> MSDILQELLRVSEKAANIARACRQQETLFQLLIEEKKEGEKNKKFAV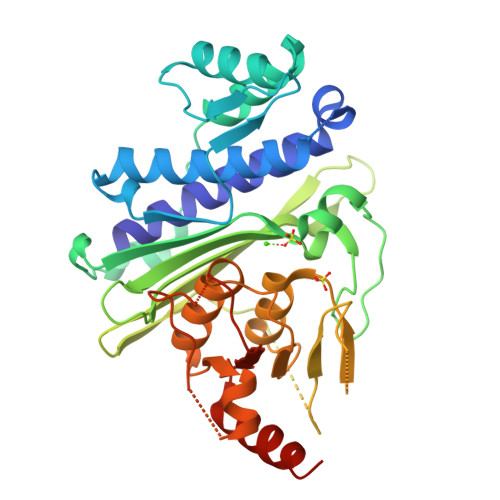DFKTLAAVLVQEVIKENMENKFPGLGKKIFGEESNELTNDLGEKIIMRLGPTEEETVALLSKVLNGNKLASEALAKVVHQDVFFSDPALDSVEINIPQDILGIWVDPIDSTYQYIKGSADITPNQGIFPSGLQCVTVLIGVYDIQTGVPLMGVINQPFVSQDLHTRRWKGQCYWGLSYLGTNIHSLLPPVSTRSNSEAQSQGTQNPSSEGSCRFSVVISTSEKETIKGALSHVCGERIFRAAGAGYKSLCVILGLADIYIFSEDTTFKWDSCAAHAILRAMGGGMVDLKECLERNPDTGLDLPQLVYHVGNEGAAGVDQWANKGGLIAYRSEKQLETFLSRLLQHLAPVATHT>[3x]VRSSSRTP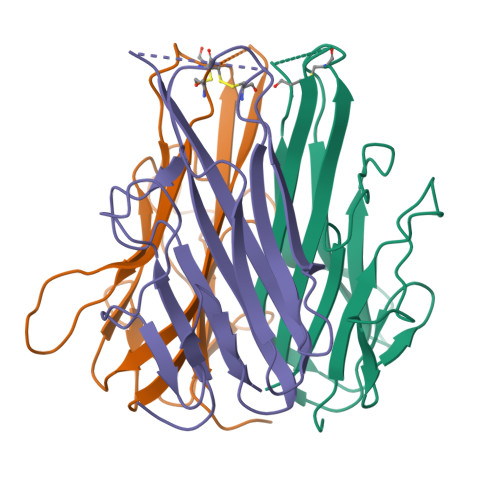SDMPVAHVVANPQAEGQLQWLNRRANALLANGVELRDNQLVVPSEGLYLIYSQVLFSGQGCPSTHVLLTHTISRITPAINRPVNLLSAIRSPCQRETPEGAEANPWYEPIYLGGVFQLEPGDRLSAEINRPDYLDFAESGQVYFGIIAL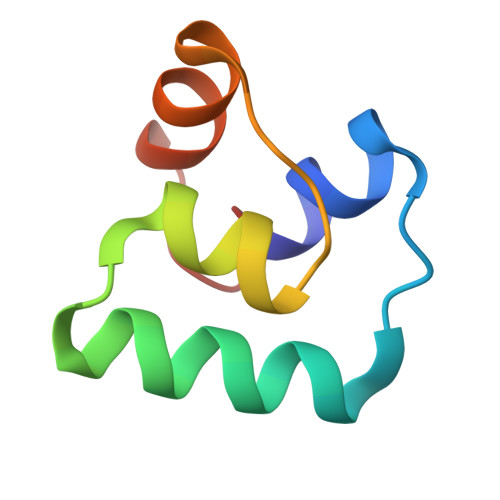>[2x]IVWIARQFGVHLTTKLTQKALDLLSSGASLGTVAAVILGVTLPGWAVAAAGALGGTAA>[2x]SWCLSVHQPWASLLVRGIKRVEGRSWYTPHRGRLWIAATAKKPSPQEVSELQATYRLLRGKDVEFPN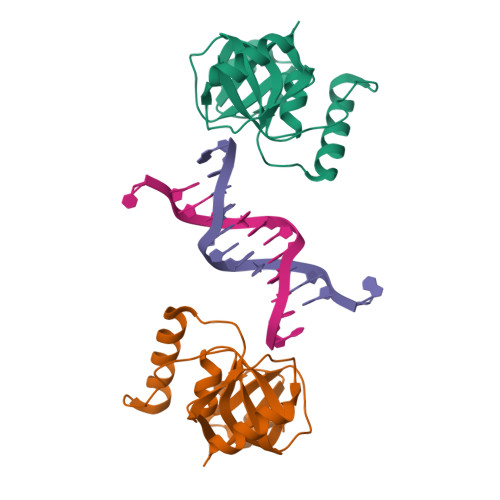DYPSGCLLGCVDLIDCLSQKQFKEQFPDISQESDSPFVFICKNPQEMVVKFPIKGNPKIWKLDSKIHQGAKKGLM>EFEC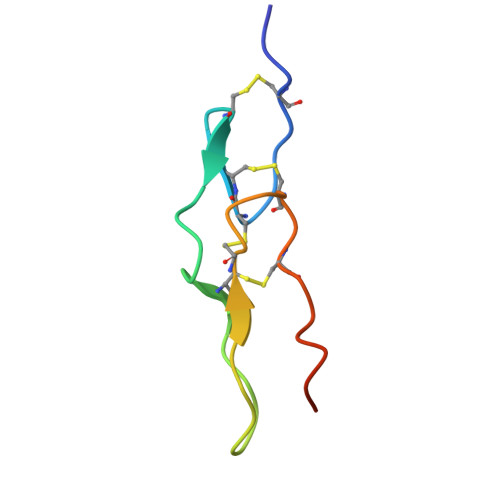ESGPCCRNCKFLKEGTICKRARGDDMDDYCNGKTCDCPRNPHKGPAT[2x]> GPAKQYDSVECPFCDEVSKYEKLAKIGQGTFGEVFKARHRKTGQKVALKKVLMENEKEGFPITALREIKILQLLKHENVVNLIEICRTKASPYNRCKGSIYLVFDFCEHDLAGLLSNVLVKFTLSEIKRVMQMLLNGLYYIHRNKILHRDMKAANVLITRDGVLKLADFGLARAFSLAKNSQPNRYTNRVVTLWYRPPELLLGERDYGPPIDLWGAGCIMAEMWTRSPIMQGNTEQHQLALISQLCGSITPEVWPNVDNYELYEKLELVKGQKRKVKDRLKAYVRDPYALDLIDKLLVLDPAQRIDSDDALNHDFFWSDPMPSDLKGMLSTHLTSMFEYLAPPRRKGSQITQQSTNQSRNPATTNQTEFERVF;> GPEGERKNNNKRWYFTREQLENSPSRRFGVDPDKELSYRQQAANLLQDMGQRLNVSQLTINTAIVYMHRFYMIQSFTRFPGNSVAPAALFLAAKVEGQPKKLEHVIKVAHTCLHPQESLPDTRSEAYLQQVQDLVILESIILQTLGFELTIDHPHTHVVKCTQLVRASKDLAQTSYFMATNSLHLTTFSLQYTPPVVACVCIHLACKWSNWEIPVSTDGKHWWEYVDATVTLELLDELTHELLQILEKTPNRLKRIWNWR

CDK9, the kinase of positive transcription elongation factor b (P-TEFb), stimulates transcription elongation by phosphorylating RNA polymerase II and transcription elongation factors. CDK9 adopts a typical protein kinase fold, whereas cyclin T has a canonical cyclin structure. In addition to the protein kinase fold, CDK9 has a C-terminal tail (residues 331–372) with a largely nonconserved sequence. Using kinetic analysis of a human P-TEFb complex consisting of CDK9 and cyclin T, we show that the CDK9 C-terminal tail sequence is important for the catalytic mechanism and imposes an ordered binding of substrates and release of products.

By soaking DRB into preformed CDK9FL/cyclin T259 crystals, we aimed to exploit this stabilizing effect to observe the CDK9 C-terminal tail residues. The resulting crystal structure, solved at 3.6 Å resolution, shows unambiguous electron density for the inhibitor and 11 additional CDK9 C-terminal residues as compared with the structure of CDK9FL/cyclin T259. CDK9 adopts a closed state upon DRB binding in which the N-terminal lobe is rotated by 8° with respect to the apo or ATP-bound structure. The CDK9 C-terminal sequence makes no direct contacts with DRB. Phe336 inserts into a hydrophobic pocket just before the hinge, and Glu337 inserts into the ATP binding site. The orientation of the CDK9 N- and C-terminal lobes induced by DRB binding is characteristic of protein kinase and protein kinase/substrate complexes that are poised for catalysis. Taken together, our results suggest that the bound state of the C-terminal tail and the associated kinase conformation observed in the CDK9FL/cyclin T259/DRB complex represents a conformation that is adopted during the reaction cycle. We propose that the DRB-bound structure of CDK9/cyclin T reported here represents a short-lived conformational state that is adopted during the phosphorylation cycle. The C terminus transiently folds over the ATP binding site, thereby stabilizing the N- and C-terminal kinase lobes and promoting ATP binding.> MAGRARSGLLLLLLGLLALQSSCLAFRSPLSVFKRFKETTRSFSNECLGTIGPVTPLDASDFALDIRMPGVTPKESDTYFCMSMRLPVDEEAFVIDFKPRASMDTVHHMLLFGCNMPSSTGSYWFCDEGTCTDKANILYAWARNAPPTRLPKGVGFRVGGETGSKYFVLQVHYGDISAFRDNHKDCSGVSVHLTRVPQPLIAGMYLMMSVDTVIPPGEKVVNADISCQYKMYPMHVFAYRVHTHHLGKVVSGYRVRNGQWTLIGRQNPQLPQAFYPVEHPVDVTFGDILAARCVFTGEGRTEATHIGGTSSDEMCNLYIMYYMEAKYALSFMTCTKNVAPDMFRTIPAEANIPIPVKPDMVMMHGHHKEAENKEKSALMQQPKQGEEEVLEQGDFYSLLSKLLGEREDVHVHKYNPTEKTESGSDLVAEIANVVQKKDLGRSDAREGAEHEEWGNAILVRDRIHRFHQLESTLRPAESRAFSFQQPGEGPWEPEPSGDFHVEEELDWPGVYLLPGQVSGVALDSKNNLVIFHRGDHVWDGNSFDSKFVYQQRGLGPIEEDTILVIDPNNAEILQSSGKNLFYLPHGLSIDTDGNYWVTDVALHQVFKLDPHSKEGPLLILGRSMQPGSDQNHFCQPTDVAVEPSTGAVFVSDGYCNSRIVQFSPSGKFVTQWGEESSGSSPRPGQFSVPHSLALVPHLDQLCVADRENGRIQCFKTDTKEFVREIKHASFGRNVFAISYIPGFLFAVNGKPYFGDQEPVQGFVMNFSSGEIIDVFKPVRKHFDMPHDIVASEDGTVYIGDAHTNTVWKFTLTEKMEHRSVKKAGIEVQEIKEAEAVVEPKVENKPTSSELQKMQEKQKLSTEPGSGVSVVLITTLLVIPVLVLLAIVMFIRWKKSRAFGDHDRKLESSSGRVLGRFRGKGSGGLNLGNFFASRKGYSRKGFDRVSTEGSDQEKDEDDGTESEEEYSAPLPKPAPSS

Two enzymes, peptidylglycine α-hydroxylating monooxygenase (PHM; EC 1.14.17.3) and peptidyl-α-hydroxyglycine α-amidating lyase (PAL; EC 4.3.2.5) working sequentially are the only proteins known to catalyze this reaction. PHM, a two Cu enzyme, catalyzes the stereospecific hydroxylation of the glycine Cα of peptidylglycine substrates. The two copper atoms in PHM, CuH, and CuM (located in the N- and C-subdomains, respectively), each use a single reducing equivalent from ascorbate to catalyze the reduction of molecular oxygen for the hydroxylation of the Cα of glycine at the carboxy-terminus of the peptide substrate. Crystallographic data on apo wild-type PHM and on several crystal forms of three CuH mutants (H107A, H108A, and H172A) presented here show that the copper ions are required not only for the catalytic steps but also for substrate binding and for locking the overall conformation of PHM in a configuration that is catalytically active.

To determine whether copper at both sites is required to bind peptide substrate, crystals of apo-PHM were both soaked and co-crystallized in mother liquor containing N-Ac-di-I-YG. This peptide binds to wild-type holo-PHM in both the oxidized and the reduced forms. In contrast, the structure of apo-PHM determined with data collected from the N-Ac-di-I-YG soaked or co-crystallized crystals showed no additional density corresponding to the bound peptide, indicating that copper at both sites is required not only for the later steps of the catalysis but also for binding substrate.> GAGCGACCTGTACGGACATCA;> AACCTACCTGGCAGGACGACT;> CACGAGC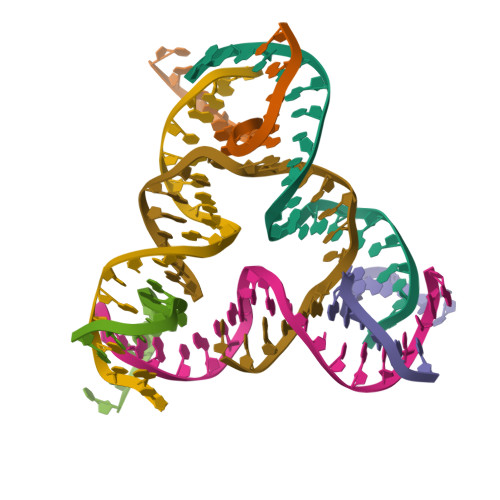CTGATCGGACAAGA;> TCTGATGTGGTAGG;> TGTCTTGTGGTCGC;> TTAGTCGTGGCTCG;> CTGCCACCGTACACCGATCA>[2x]MRGSHHHHHHGSKLTVVGLGYIGLPTSIMFAKHGVDVLGVDINQQTIDKLQNGQISIEEPGLQEVYEEVLSSGKLKVSTTPE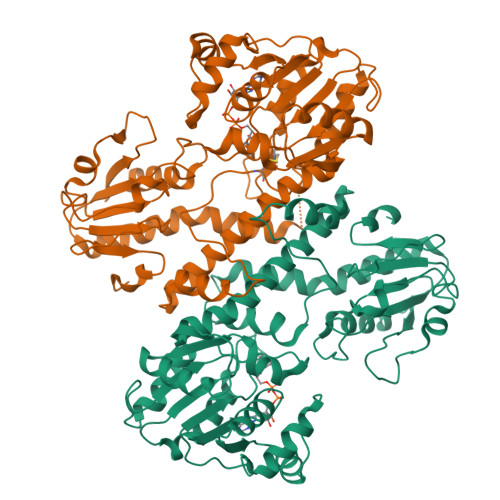ASDVFIIAVPTPNNDDQYRSCDISLVMRALDSILPFLKKGNTIIVESTIAPKTMDDFVKPVIENLGFTIGEDIYLVHCPERVLPGKILEELVHNNRIIGGVTKACIEAGKRVYRTFVQGEMIETDARTAEMSKLMENTYRDVNIALANELTKICNNLNINVLDVIEMANKHPRVNIHQPGPGVGGHCLAVDPYFIIAKDPENAKLIQTGREINNSMPAYVVDTTKQIIKALSGNKVTVFGLTYKGDVDDIRESPAFDIYELLNQEPDIEVCAYDPHVELDFVEHDMSHAVKDASLVLILSDHSEFKNLSDSHFDKMKHKVIFDTKNVVKSSFEDVLYYNYGNIFNFIDK>SMAMFYAHALGGYDENLHAFPGISSTVANDVRKYSVVSVYNNKYDIVKDKYMWCYSQVNKRYIGALLPMFECNEYLQIGDPIHDQEGNQISIITYRHKNYYALSGIGYESLDLCLEGVGIHHHVLETGNAVYGKVQHDYSTIKEKA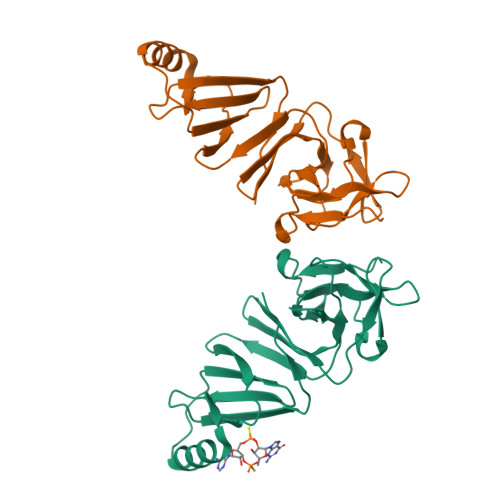KEMNALSPGPIIDYHVWIGDCICQVTAVDVHGKEIMRMRFKKGAVLPIPNLVKVKLGENDTENLSSTISAAPSR[10x]> GGAPWQAEEWYFGKITRRESERLLLNAENPRGTFLVREGQSQPDYVLSVSDFDNAKGLNVKHYIIRKLD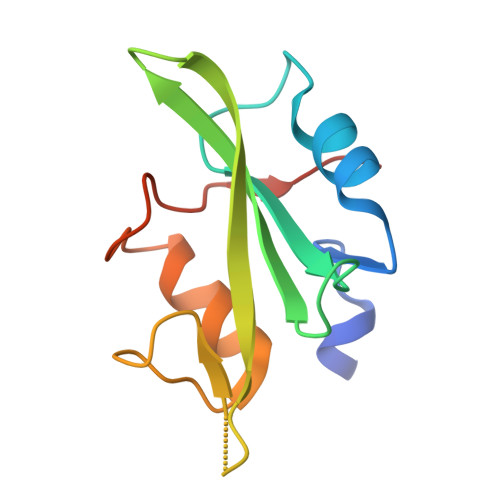SGGFYITSRTQFNSLQQLVAYYSKHADGLCHRLTTVCPTSRA> GSGAMAQNLDSMLHGTGMKSDSDQKKS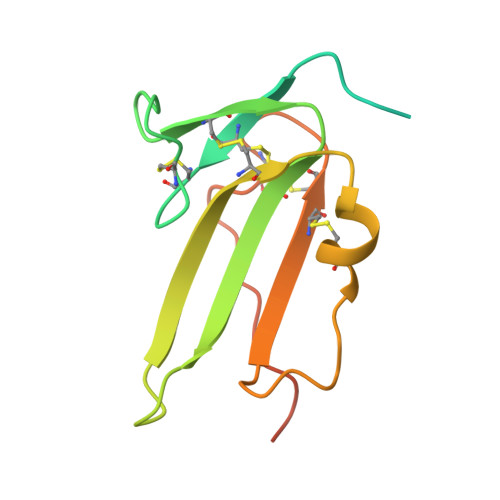ENGVTLAPEDTLPFLKCYCSGHCPDDAINNTCITNGHCFAIIEEDDQGETTLASGCMKYEGSDFQCKDSPKAQLRRTIECCRTNLCNQYLQPTLPPVVIGPFFDGSIR>[4x]MEIRYTPKELTKLPRTVEYKNKSVYMINQRLLPKEFKVEKFSKVEEVAEAIKNMTVRGAPAIGAAAG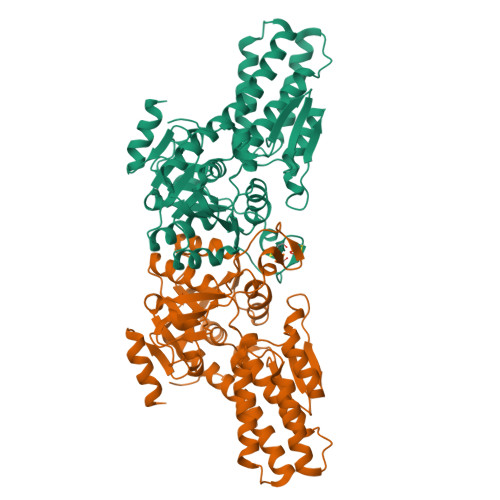FGLALYAETSKAKTKEEFLDGFEKAYEILKNTRPTAVNLFWALNRIKKLVEEHSEDPLDEIKRLIVQEAYKIADEDVEANLRMGHYGAEVLPEGNILTHCNAGSLATVHLGTVGSVVRVMHKDGSLKLLWLDETRPVLQGARLSAWEYSYDGLNVKLIADNAAAFVMQQGFVDAIIVGADRIVANGDFANKIGTYMLAVLAREHGIPFFAVAPLSSIDMELKSGKDIPIEERSPEEVLTCGGCRIAPDVPVYNPAFDVTPHKYLTGIITDRGVVWPPFKRNLKKLFEVNKSGGDEAV> GSMVEATAQETDRPRFSFSIAAREGKARTGTIEMKRGVIRTPAFMPVGTAATVKALKPETVRATGADIILGNTYHLMLRPGAERIAKLGGLHSFMGWDRPILTDSGGYQVMSLSSLTKQSEEGVTFKSHLDGSRHMLSPERSIEIQHLLGSDIVMAFDECTPYPATPSRAASSMERSMRWAKRSRDAFDSRKEQAENAALFGIQQGSVFENLRQQSADALAEIGFDGYAVGGLAVGEGQDEMFRVLDFSVPMLPDDKPHYLMGVGKPDDIVGAVERGIDMFDCVLPTRSGRNGQAFTWDGPINIRNARFSEDLKPLDSECHCAVCQKWSRAYIHFLIRAGEILGAMLMTEHNIAFYQQLMQKIRDSISEGRFSQ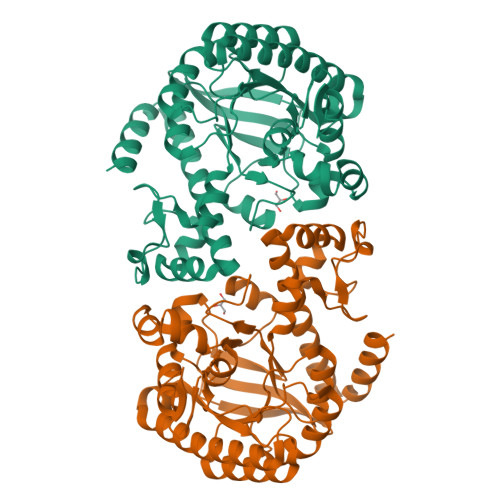FAQDFRARYFARNS> MLSFLGKSVALLAALQATLSSPKPGHRRASVEKRANGYANSVYFTNWGIYDRNFQPADLVASDVTHVIYSFMNLQADGTVISGDTYADYEKHYADDSWNDVGTNAYGCVKQLFKVKKANRGLKVLLSIGGWTWSTNFPSAASTDANRKNFAKTAITFMKDWGFDGIDIAWAYPADATQASNMILLLKEVRSQLDAYAAQYAPGYHFL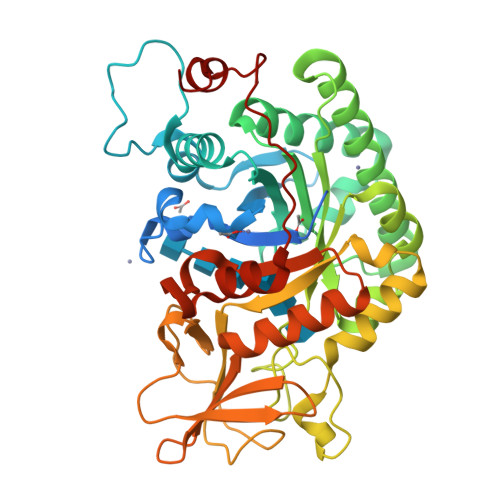LTIAAPAGKDNYSKLRLADLGQVLDYINLMAYDYAGSFSPLTGHDANLFNNPSNPNATPFNTDSAVKDYINGGVPANKIVLGMPIYGRSFQNTAGIGQTYNGVGSGSWEAGIWDYKALPKAGATVQYDSVAKGYYSYNSATKELISFDTPDMINTKVAYLKSLGLGGSMFWEASADKKGADSLIGTSHRALGGLDTTQNLLSYPNSKYDNIKNGLN>HMSIMKVYCQICRKGDNEELLLLCDGCDKGCHTYCHRPKITT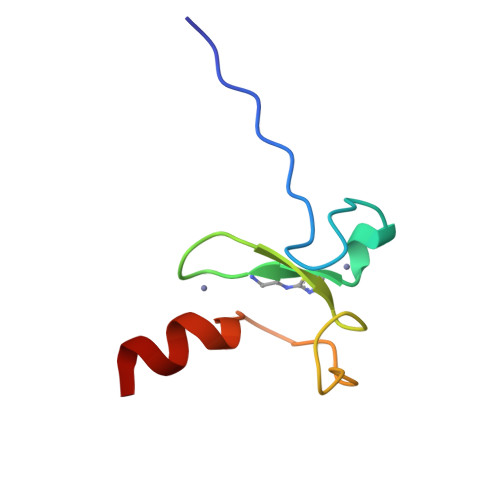IPDGDWFCPACIAKAS[2x]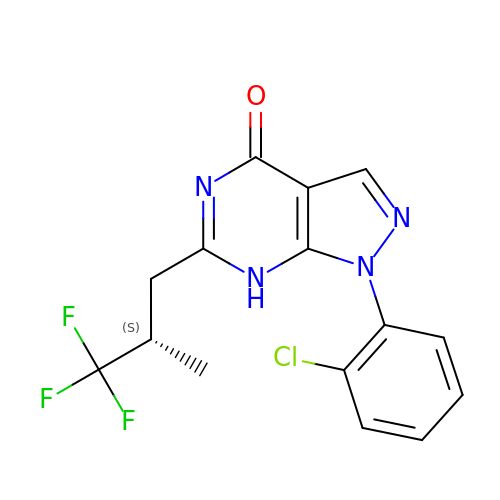1-(2-chlorophenyl)-6-[(2S)-3,3,3-trifluoro-2-methylpropyl]-1,7-dihydro-4H-pyrazolo[3,4-d]pyrimidin-4-one | C15 H12 Cl F3 N4 O | FFPXPXOAFQCNBS-QMMMGPOBSA-N>GKAFDDGAFTGIREINLSYNKETAIGDFQVVYDLNGSPYVGQNHSSFISGFTPVKISLDFPSEYITEVSGYTGNVSGYVVVRSLTFKTNKKTYGPYGVTSGTPFNLPIENGLIVGF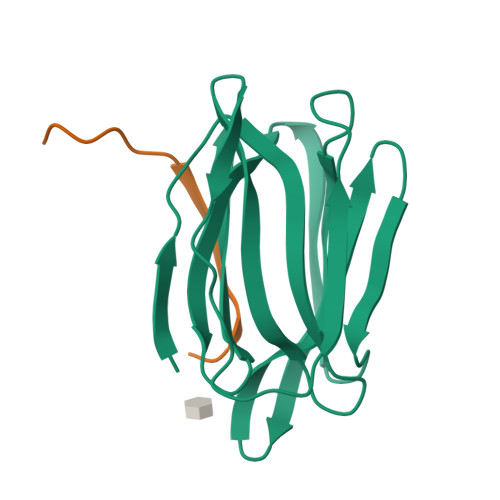KGSIGYWMDYFSMYLSL[4x];>[4x]DENSGKSQTVIVGPWGAKVS>[4x]MPKSTYFSLSDEKRNRVYDACLN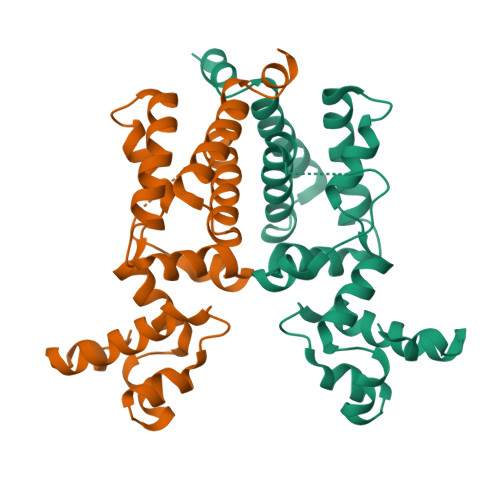EFQTHSFHEAKIMHIVKALDIPRGSFYQYFEDLKDAYFYVLSQETLEIHDLFFNLLKDNSIEESLDKYKYLLLENLIDSPQYKLYKYRFLDWTYELERDWKPQSSATVPASENDNPISQVLKSVVHNLVYRLFSENWTEKTFIENYDKEIKLVTEGLLNYITDRKN>[3x]PAIQSELDVNGEDFARNREAMLAAVAGFRELEQKVLDKAAEARPKFEKRGQLLPRERLALLLDPGAPFLELSSLAGYKLHDDKDGTQAGGGIIAGIGYIAGVRCLVSASNSAIKGGTISPTGLKKTLRLQQIAMENKLPVVTLTESGGANLNYAAEIFVEGARGFANQARISAMGIPQVTVVHGSSTAGGAYQPGLSDYVVVVRGKAKMFLAGPPLLKAATGEIASDEELGGAELHAQVAGTAEYLAENDADGVRLAREIVGMLPWNAQLPARPARSWREPLYPVEELLGVVPADPKKPYDVREIVARIADGSEFLDFKNEFDGQTVCGHLRIEGHACGLIGNNGPITPQGAAKAAQFIQLCEQSNTPLLFLHNTTGFMVGTESERQGVIKHGSKMIQAVANARVPKLTLVVGGSYGAGNYAMCGRGLDPRFIFAWPNSRTAVMGGAQAGKVLRIVTEEKHAKEGKEADPKMLEMLETVTAQK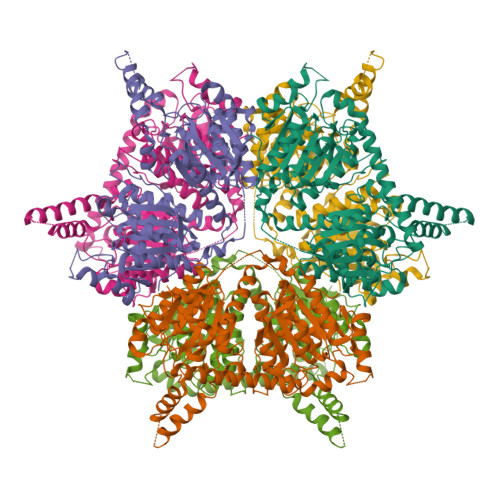LDSQSTALYGTASLWDDGLVDPRDSRRLLGYLLDICAEAEARPLKGNSFGVARF>AADEPQLLHGAGICKWFNVRMGFGFLSMTARAGVALDPPVDVFVHQSKLHMEGFRSLKEGEAVEFTFKKSAKGLESIRVTGPGGVFCIGSERRPKGGDRCYNCGGLDHHAKECKLPPQPKKCHFCQSINHMVASCPLKA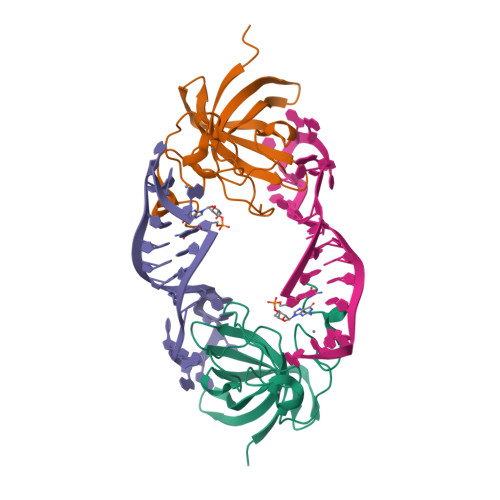QQGPSSQGK[2x]>[3x]TGPYAGAVEVQQSGRYYVPQGRTRGGYINSNIAEVCMDAGAAGQVNALLAPRRGDAVMIYFVWRPLRIFCDPQGASLESAPGTFVTVDGVNVAAGDVVAWNTI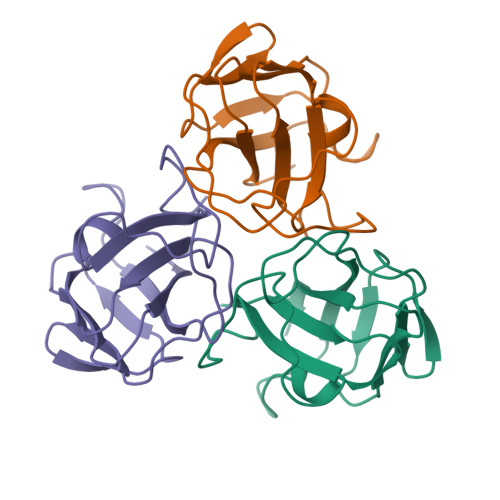APVNVGNPGARRSILQFEVLWYT> MARTPQEVLKWIQDENIKIIDLKFIDTPGIWQHCSFYYDQLDENSFTEGIPFDGSSIRGWKAINESDMCMVPDPNTATIDPFCKEPTLSMICSIKEPRTGEWYNRDPRTIAAKAAEYLRGTGIADTVYFGPEAEFFLFDDIRF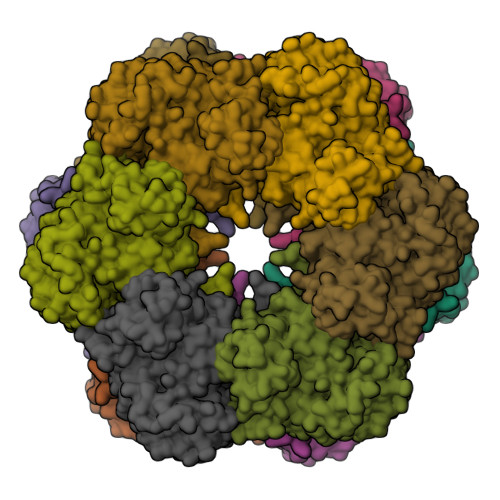GQTENSSYYFADSVEGRWNTGREEEGGNLGYKPGYKQGYFPVAPTDTAQDIRTEMLLTMAAFGVPIEKHHHEVASGGQNELGIKFDKLVNSADNLMIYKYVIKNVAKKYGKTVTFMPKPIFNDNGSGMHVHQSLWKDGQPLFAGDKYAGFSQMGLWYIGGILKHAPALLAFTNPTTNSYKRLVPGFEAPVNLAYSQGNRSASVRIPLSGGNPKAKRLEFRCPDATSNPYLAFAAMLCAGIDGIKNQIDPGEPLDVDIYDLSPEELAKIPSTPGSLEAALEALEKDHEFLTGTGVFSPDFVESWIEYKLDNEVNPMRLRPHPYEFSLYYDC>MTSVSVAFTNVAGLLAHGSKSRCRNAEVLRSRSAAERASGDRQRWRICMSDGERVHAYTETVVESQLGFSVSRRALLHHLALGALAVALPRSGALVAAPLAETVRGAAWKQVPLPTESVLFDIDFSQKDPNHGWLVGTRGLVLETRDGGETWEPR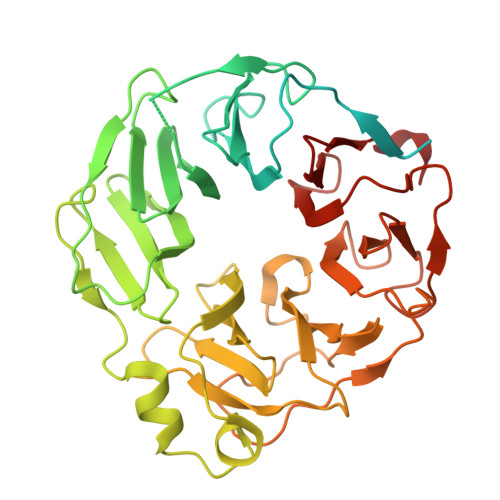AFEDVEREEELNYRFSNVSFSGDEAWVIGKPPVMLRSTDGGKNWSRILLSPKLPGEPLLVTALGPNCAEMVTSSGAIYVTENGGINWKALVRETIDATLNRTISSGITGASYFTGSIVSVSRDVHGNYIAIPSRGNFFLTWVPGSDFWTPHARSTSRRISAIGFIQNDATKGIWETIRGGGLGFTKPNVNLNSTETIAFDMVDSKTGGYGILDVAFQDDRHVWAAVGGGSMYRSDDGGKTWRRDPLVSKVGANLYKIKFFGSQRGFVLGADGVLLKFHPENV[2x]>SRETRYVELYVVVDNAEFQMLGSEAAVRHRVLEVVNHV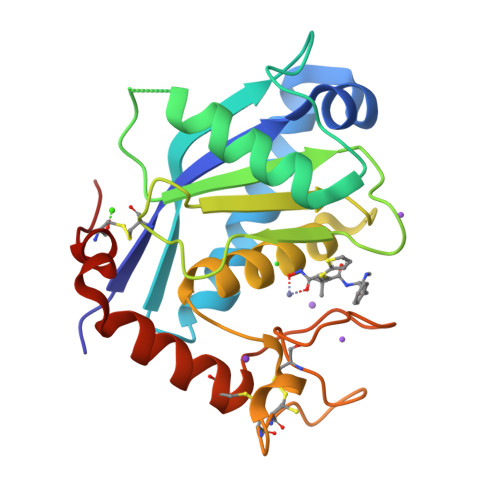DKLYQKLNFRVVLVGLEIWNSQDRFHVSPDPSVTLENLLTWQARQRTRRHLHDNVQLITGVDFTGTTVGFARVSAMCSHSSGAVNQDHSKNPVGVACTMAHEMGHNLGMDHDENVQGCRCQERFEAGRCIMAGSIGSSFPRMFSDCSQAYLESFLERPQSVCLANAPDLS[4x]> HHHHHHMDIIFYHPTFDTQWWIEALRKAIPQARVRAWKSGDNDSADYALVWHPPVEMLAGRDLKAVFALGAGVDSILSKLQAHPEMLNPSVPLFRLEDTGMGEQMQEYAVSQVLHWFRRFDDYRIQQNSSHWQPLPEYHREDFTIGILGAGVLGSKVAQSLQTWRFPLRCWSRTRKSWPGVQSFAGREELSAFLSQCRVLINLLP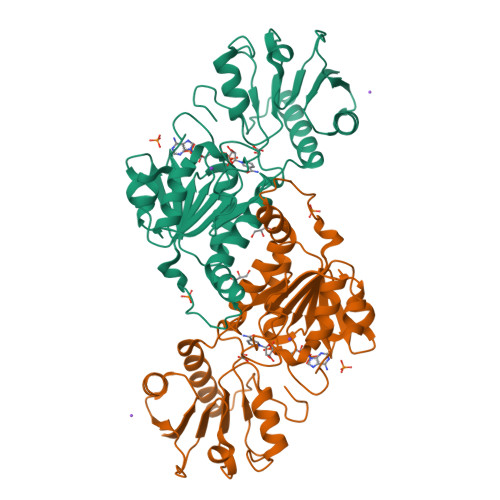NTPETVGIINQQLLEKLPDGAYLLNLARGVHVVEDDLLAALDSGKVKGAMLDVFNREPLPPESPLWQHPRVTITPHVAAITRPAEAVEYISRTIAQLEKGEKVCGQVDRARGY> MKSESKVSSKLELRELVLLAMVIAIKVILGQFKVGNATLQVGLGFIGSVMLGYLFGPWWGFAGGALSDLVSSVIFGNLGGFFIGFTLTAALGPMIYGFFLYKQPIQIWRVIASVICVTVICNIGLNTLWVSMMYGINFMVALSSRILKEMITPWI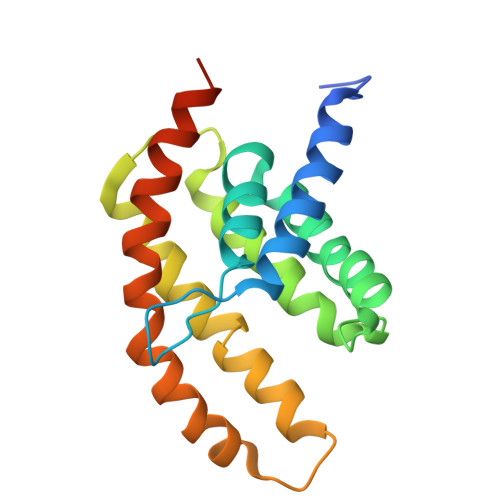QMVAVWFILEGLSRVKLSRKFWSHPQFEK>[4x]GSAAAGHRTVYLFDRREKESELGDRPLQVGERSDYAGFRACVCQTLGISPEEKFVITTTSRKEITCDNFDETVKDGVTLYLLQSVNQLLLTATKERIDFLPHYDTLVKSGMYEYYASEGQNPLPFALAALIDNSLSATSRNIGVRRIQIKLLFDETQGKPAVAVIDNGRGMTSKQLNNWAVYRLSKFTRQGDFESDHSGYVRPVPVPRSLNSDISYFGVGGKQAVFFVGQSARMISKPADSQDVHELVLSKEDFEKKEKNKEAIYSGYIRNRKPSDSVHITNDDERFLHHLIIEEKEKDSFTAVVITGVQPEHIQYLKNYFHLWTRQLAHIYHYYIHGPKGNEIRTSKEVEPFNNIDIEISMFEKGKVPKIVNLREIQDDMQTLYVNTAADSFEFKAHVEGDGVVEGIIRYHPFLYDRETYPDDPCFPSKLKDEDDEDDCFILEKAARGKRPIFECFWNGRLIPYTSVEDFDWCTPPKKRGLAPIECYNRISGALFTNDKFQVSTNKLTFMDLELKLKDKNTLFTRILNGQEQRMKIDREFALWLKDCHEKYDKQIKFTLFK

Structural maintenance of chromosomes hinge-domain containing protein 1 (SMCHD1), an emerging player in the field of epigenetics, is a unique member of the GHKL superfamily. Originally identified in a mutagenesis screen for novel epigenetic repressors of repeat sequences, SMCHD1 is now known to not only silence repeats but also a subset of autosomal genes, particularly those that are imprinted, mono-allelically expressed, or clustered, and to maintain X-chromosome inactivation. SMCHD1 is a 2005aa protein with an N-terminal functional GHKL-ATPase module (1–578aa), an extended non-conserved middle region of unknown function, and a C-terminal SMC-hinge domain (1616–1963aa) that mediates constitutive dimerization. Herein, we have revealed the crystal structure of the SMCHD1 N-terminal module which contains all of the conserved elements of the Bergerat ATP-binding fold, a transducer domain, and a novel ubiquitin-like (UBL) fold.

The crystal structure of the GHKL-ATPase module in the presence of ATP was solved at 2.2 Å by expressing a construct consisting of residues 24–580 with a E147A inactivating variant. The asymmetric unit contains two dimers which adopt similar conformations (RMSD of 0.71 Å over 972 Cαs). Each monomer is comprised of three domains: a pre-N terminal domain with a ubiquitin-like fold (UBL) (25–109aa), a GHKL-ATPase catalytic domain (110–395aa), and a transducer domain (396–578aa). ATP bound to the active site is stabilized by interactions with residues from each of these motifs and by an octahedrally coordinated Mg2+ ion that forms interactions with oxygens from each of the three phosphate groups of ATP and with the conserved Asn151 from Motif I on α-helix 4. The proposed catalytic base, Glu147 (mutated to Ala in the crystal structure to inhibit ATP hydrolysis), is also located within Motif I on the same central α-helix as Asn151. In the SMCHD1 crystal structure, the ATP lid exists in a closed conformation and is located between Motif II and Motif III and extends into Motif III. A loop between β-strand 17 and α-helix 15, termed the “switch-loop”, extends from the central domain structure along the dimer interface and positions Lys525 at the ATP binding site for a hydrogen bond with the γ-phosphate. The SMCHD1(24–580/E147A) construct forms the canonical GHKL-ATPase dimer with an N-terminal β-strand (110–120aa) “strap” that is swapped between monomers. One unique feature of the N-terminal domain swap in SMCHD1 compared with other GHKL-ATPases is the addition of a UBL domain. SMCHD1 N-terminal dimerization generates a cavity between the transducer domains of the two monomers that is flanked on both sides by a disordered loop (447–463aa).> EDSKLSIISWNVDGLDTLNLADRARGL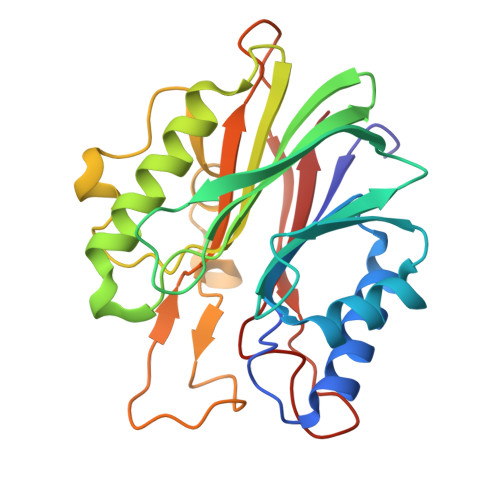CSYLALYTPDVVFLQELIPAYVQYLKKRAVSYLFFEGSDDGYFTGIMLRKSRVKFLESEIICFPTTQMMRNLLIAQVTFSGQKLYLMTSHLESCKNQSQERTKQLRVVLQKIKEAPEDAIVIFAGDTNLRDAEVANVGGLPAGVCDVWEQLGKQEHCRYTWDTKANSNKTVPYVSRCRFDRIFLRSAKTAPPVTPDHMALIGMEKLDCGRYTSDHWGIYCTFNT> GSMSGPVTYTHDDAI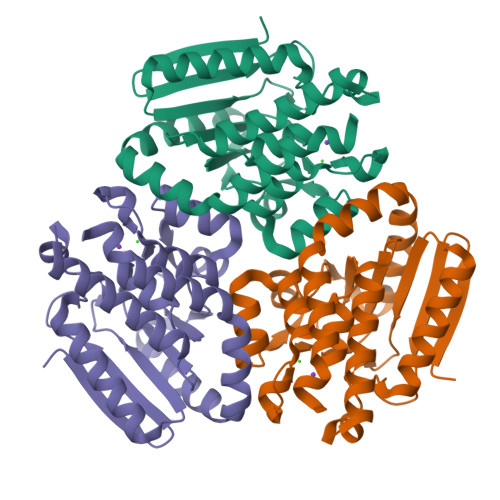GVIRMDDGKVNVLGPTMQQALNEAIDAADRDNVGALVIAGNHRVFSGGFDLKVLTSGEAKPAIDMLRGGFELSYRLLSYPKPVVIACTGHAIAMGAFLLCSGDHRVAAHAYNVQANEVAIGMTIPYAAMEVLKLRLTPSAYQQAAGLAKTFFGETALAAGFIDEISLPEVVLSRAEEAAREFAGLNQQAHNATKLRARAEALKAIRAGIDGIEAEFGL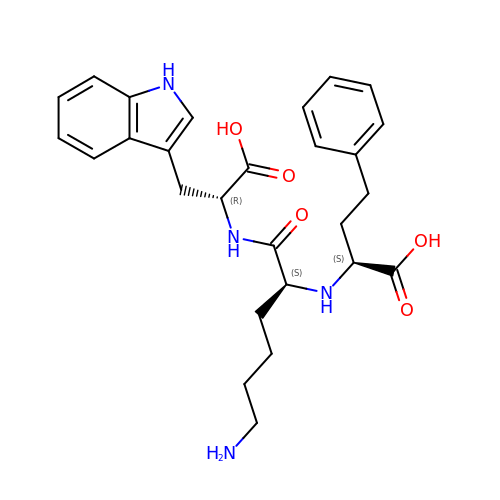(S)-1-N2-(1-CARBOXY-3-PHENYLPROPYL)-L-LYSYL-L-TRYPTOPHAN | C27 H34 N4 O5 | JXNGDSIPMBNTNL-KMDXXIMOSA-N>[2x]GAGDVVTRDVNKLPVAAREMIGKHFSQTKVAYIKIEKDLFQTTSYDVKLADGIELEFNSKGEWLEIDCKNKSVP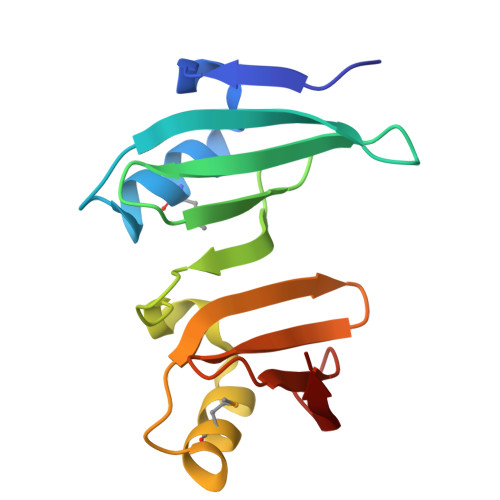STFIPQAISKYMKANYNGHKTVKIERNRKGYELTLENGLEVDFDQFGGFLKLSD>[2x]ASAWPEEKNYHQPAILNSSALRQIAEGTSISEMWQNDLQPLLIERYPGSPGSYAARQHIMQRIQRLQADWVLEIDTFLSQTPYGYRSFSNIISTLNPTAKRHLVLACHYDSKYFSHWNNRVFVGATDSAVPCAMMLELARALDKKLLSLKTVSDSKPDLSLQLIFFDGEEAFLHWSPQDS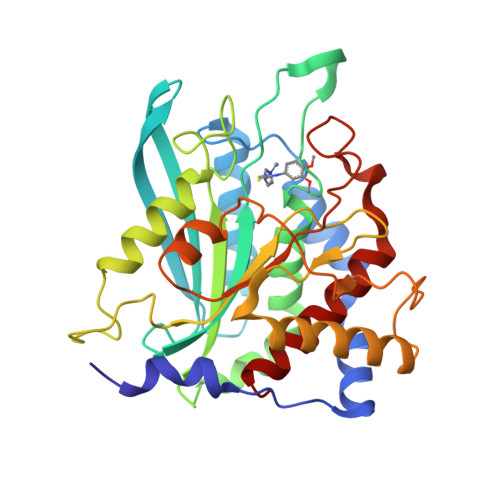LYGSRHLAAKMASTPHPPGARGTSQLHGMDLLVLLDLIGAPNPTFPNFFPNSARWFERLQAIEHELHELGLLKDHSLEGRYFQNYSYGGVIQDDHIPFLRRGVPVLHLIPSPFPEVWHTMDDNEENLDESTIDNLNKILQVFVLEYLHL>GMADSASQAEQFLKLVHADKLTVPVYAQVQQMLAQRFAQAKAPESKKAVLERYQAKANAELDRAIGWDKIKPELIKLYTTNFTESELKDLNAFYQSPLGKKVLEKMPRLTAESAQ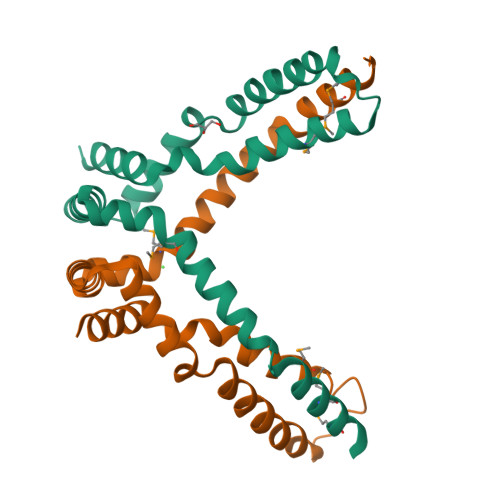LTQAKLQGAVEPVNKLMADMDKELGVAAPAQKKK[2x]>[112x]MGLFDRIKRVVSSNLNDLVNKAEDPEKMLEQAILEMQEDL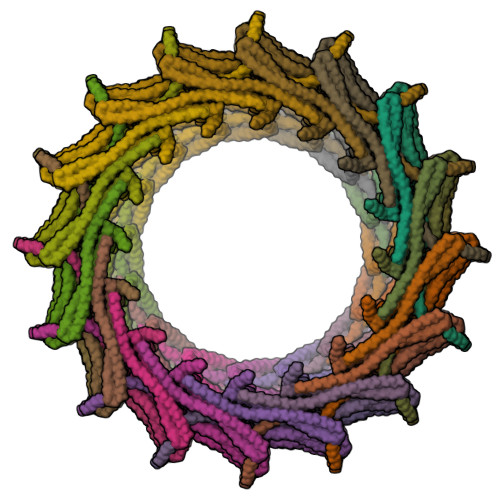VQLRQGVAQAIAAQKRSEKQYNDAQNEINKWQRNAQLALQKGDENLARQALERKKTYTDTSAALKASLDTQSTQVETLKRNLIQLESKISEAKTKKEMLKARITTAKAQEQLQGMVRGMNTSSAMSAFERMEEKVLMQESRAQALGELAGADLETQFAQLEGGSDVDDELAALKAQMLPPATPVTQAQLPPQQETTPAKSNEVVDAELDSLRKQLDQL>GGCG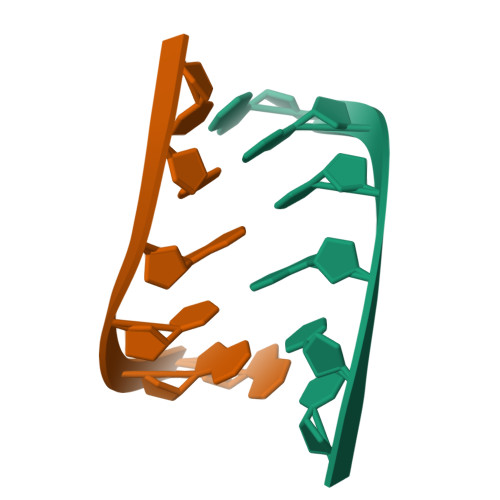CC[6x]>HVRSYNHLQGDVRWRKLFSFTKYFLKIEKNGKVSGTKKENCPYSILEITSVEIGVVAVKAINSNYYLAMNKKGKLYGSKEFNNDCKLKERIEENGYNTYA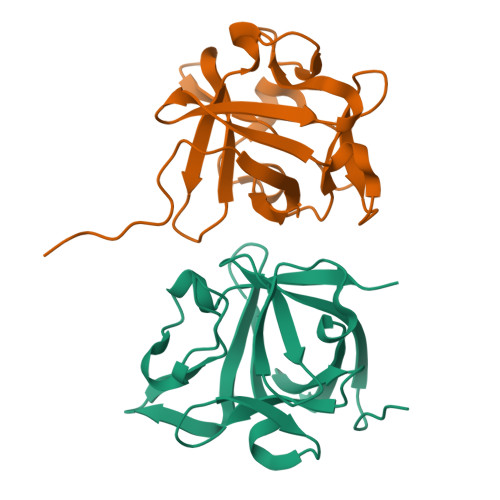SFNWQHNGRQMYVALNGKGAPRRGQKTRRKNTSAHFLPMVVH[2x]Pectocin M1 (PM1), the bacteriocin from phytopathogenic Pectobacterium carotovorum which causes soft rot disease, has a unique ferredoxin domain that allows it to use FusA of the plant ferredoxin uptake system.

To probe the structure‐based mechanism of PM1 uptake, we determined the X‐ray structure of full‐length PM1, containing an N‐terminal ferredoxin and C‐terminal catalytic domain connected by helical linker, at 2.04 Å resolution. Based on published FusA structure and NMR data for PM1 ferredoxin domain titrated with FusA, we modeled docking of the ferredoxin domain with FusA. Combining the docking models with the X‐ray structures of PM1 and FusA enables us to propose the mechanism by which PM1 undergoes dynamic domain rearrangement to translocate across the target cell outer membrane.

>[4x]MATYKIKDLTGNVEFECSDDTYILDAAEEAGLDLPYSCRAGSCSSCVALLISGSVDQRDASFLDEEQQKYFVLTCAAYPNSNCVIKTGVEEMLLGYDSYRDMSEYLFGLLGGNDSPELLDGLFTPVDAFRHYLFGNGTNKSININDVGLSIDVSQIPPIMNIINQGFIGRFDISSDFNRNTVLDGIIPASYLGNITLKTEGVLSISPDGAWSYNGGIRAYNDLYDANPSTHRDRLGEWSTGVLDKFNGTPYEIQIPGTLDISGRGQRL>[6x]MHHHHHH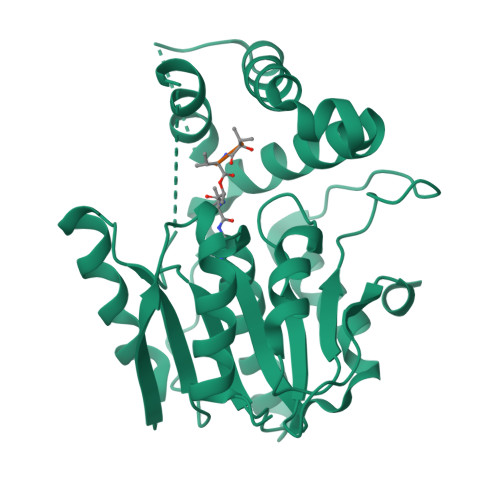HHENLYFQGGSSTAGDPTAKLVRLNPRGGDGPGIVFAPPAGGTVLGYIELARHLKGFGEIHGVEAPGLGAGETPVYPSFEEMVQFCSDSAAGVAGDGVYIGGHALGGHIAFYLATMLLDRGIRPKGLIILDTPPRLGDIPVADADLTEEETKVFILAMGIGGMLDQDRDALKDLPYEEAKQLLLDRAKNDPRVSAFLSEDYLDRFLRLQMHQLMYSRDVVLPQRKLDIPIHVFRTKNHAPEVARLFSAWENYAAGEVTFVDIPGDHATMLRAPHVSEVAQLLDRHCGLPSDDGPRG>GSPASGTSLSAA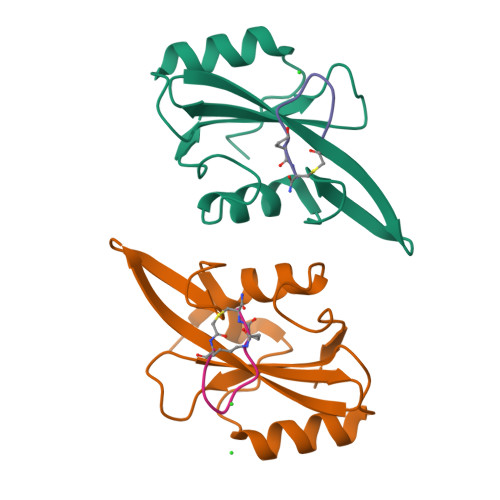IHRTQLWFHGRISREESQRLIGQQGLVDGLFLVRESQRNPQGFVLSLCHLQKVKHYLILPSEEEGRLYFSMDDGQTRFTDLLQLVEFHQLNRGILPCLLRHCCTRVAL[4x];>KFEGYDNEX[4x]> TNKPIVLSTWNFGLHANVEAWKVLSKGGKALDAVEKGV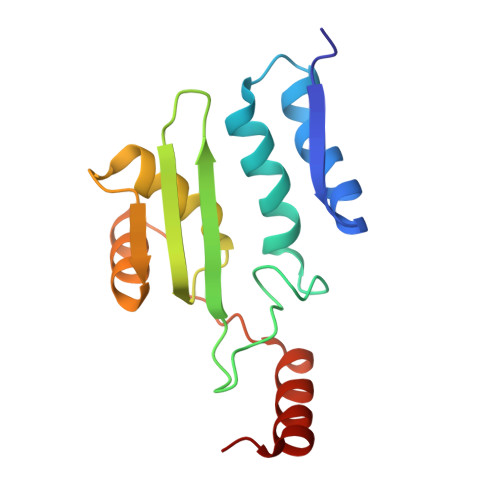RLVEDDPTERSVGYGGRPDRDGRVTLDACIMDENYNIGSVACMEHIKNPISVARAVMEKTPHVMLVGDGALEFALSQGFKKENLLTAESEKEWKEWLKTSQYK> MIVLFVDFDYFY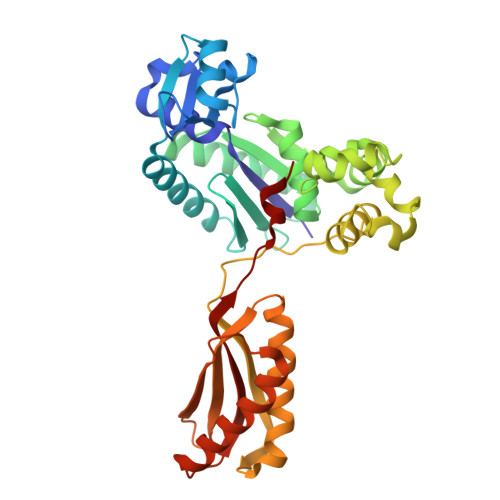AQVEEVLNPSLKGKPVVVCVFSGRFEDSGAVATANYEARKFGVKAGIPIVEAKKILPNAVYLPMRKEVYQQVSSRIMNLLREYSEKIEIASIDEAYLDISDKVRDYREAYNLGLEIKNKILEKEKITVTVGISKNKVFAKIAADMAKPNGIKVIDDEEVKRLIRELDIADVPGIGNITAEKLKKLGINKLVDTLSIEFDKLKGMIGEAKAKYLISLARDEYNEPIRTRVRKSIGRIVTMKRNSRNLEEIKPYLFRAIEESYYKLDKRIPKAIHVVAVTEDLDIVSRGRTFPHGISKETAYSESVKLLQKILEEDERKIRRIGVRFSKFIEAIGLDKFFDT>MIELRNLTKWYPTPHGRRYVFRNLNFRFPDDVSIGLIGRNGAGKSTLMRLLGGIEAPNEGEVVTDVSISWPVGLSGGFQGSLTARENVKFVCRIYGTSHEDMLRKVRFVEEFAEIGEHFDLPMKTYSSGMRSRVAFGLSMAFDFDYYLIDEAMAVGDAQFRAKSRAVFDSRVGQANMILVSHNMNDIKEYCDVVVLVDQGQATLYEDVEAGIAAYQGSLKKAAAKPDYKDDDDK[2x];>[2x]MGKIHLAVSERSPRVKRSPWQIQQAVLFALFLRELKTRLGGRWLGVFWVLLEPVAHIAVMTTLFSLAHRAAMPSIEYPVFLITGLIPFFMFRGLVTRLMEAIDSNRGLFAYRQVKPIDTVIARAMLEISLQSIVYLIALGTLGWLGFHFLPVRALELAGVSAVLIMLGASLGLFFAVVTNEIPQARAIVRISLLPLYFVSGVIFPVHTIPPQYLPLLQLNPVLHLIELSRASFFPQYRVLQGINLAYPAGFALLSLFLALMLYRLRRHQLASVV;>MGKIHMKLVSRLTAKRLQWALVYLPMLVATVYFLVFSADRYVSESVITVRQTSSNAPTGGMSGAALLLAGLTPASREDTCYLQTYIHSMGLLQKLDQQLKLREHFGTPLRDPLFRLWGGTSQEWFLEYYRSRVEVLMDDICGLLTVRVQGFEPEFAQALNRAILEESERFVNELSHRMAREQGQFAEAELERATARLQEAKRQLIAFQAKHKLLDPLAQAQATGTLTAELQAALTRQEAELRNALTYLNEDSYQVKALRSQINALRQQIDEERLRATAGKNGDRINAVAAEFHDLQLQVGFAEDAYKLALAAVESARIEATRKLKSLVVVEPPVLPEIAEYPRRWYNLATLLVVCCLIYGVVSLVVATIRDHQDGSGSGSHHHHHHHHHH[8x]

CPS secretion is mediated by an ABC transporter containing KpsT and KpsM as its nucleotide-binding domain (NBD) and transmembrane domain, respectively. The transporter partners with the periplasmic and inner-membrane-anchored KpsE subunit, a class-3 polysaccharide co-polymerase (PCP), as well as with KpsD, which is assumed to form an outer-membrane pore. The KpsMT transporter is surrounded by a cage of eight KpsE subunits extending about 80 Å into the periplasm. Cryo-electron microscopy analyses of the KpsMT–KpsE complex in six different states reveal a KpsE-encaged ABC transporter, rigid-body conformational rearrangements of KpsMT during ATP hydrolysis and recognition of a glycolipid inside a membrane-exposed electropositive canyon.

To determine how KpsMT recognizes the glycolipid, the purified KpsMT–KpsE complex was preincubated with the isolated glycolipid before cryo grid preparation. Cryo-EM analyses of this sample provided additional cryo-EM maps similar in overall architecture to the Apo 1 state, but with poorly defined KpsT subunits. However, in contrast to all other structures, we identified two states of a lipid molecule bound inside the canyon (referred to as state-1 and state-2). Therefore, we modelled the putative ligand as a phosphatidylglycerol-linked Kdo monosaccharide, with the caveat that the Kdo conformation and its interactions are not precisely resolved. In state-1, with the putative Kdo sugar closer to the cytosolic water–lipid interface, the sugar moiety is sandwiched between TM1 and TM5 of opposing KpsM protomers. Although the exact position of the Kdo moiety is speculative, it is surrounded on one side by Trp45 of TM1 and, through the opposite face of the sugar ring, Gln181, Ile185 and Ile188 of TM helix 5 of the second KpsM protomer. The following phosphate group is near Arg94 of TM2. One lipid acyl chain snakes through the hydrophobic segment of the canyon, where it is surrounded by Phe85 and Phe86 of TM2, as well as by Leu191, Tyr194 and Phe195 of TM5 of the same protomer. The second acyl chain points away from the KpsM subunits and does not mediate extensive protein interactions.>[13x]MAFLGAAIAAGLAAVAGAIAVAIIVKATIEGTTRQPELRGTLQTLMFIGVPLAEAVPIIAIVISLLILF

Most living cells depend upon the adenosine triphosphate (ATP) generated by F1Fo-ATP synthases that are energized by a proton- or a sodium-motive force (pmf, smf). Energetically down-hill ion translocation across the membrane through the Fo complex is mediated by successive interactions between the stator a-subunit and a rotor ring (c-ring). Translocation involves ion binding to an unoccupied c-subunit, rotation, and subsequent ion release. The c-ring is attached to the γε stalk subunits so that c-ring rotation causes rotation of the stalk.

We solved the crystal structure of a novel type of c-ring isolated from Bacillus pseudofirmus OF4 at 2.5 Å, revealing a cylinder with a tridecameric stoichiometry, a central pore, and an overall shape that is distinct from those reported thus far. In contrast with the distinctly hour-glass shape of the c11, K10, and c15 rotor rings, this c13 ring resembles a “tulip beer glass” appearance, in which the only slightly curved periplasmic side transitions at about the depth of the ion-binding site into a more significantly flared cytoplasmic side. While the inner helices are remarkably straight and only slightly tilted by ∼5° toward the c-ring axis (as seen from the periplasm), the outer helices are more curved and have a kink in the middle of the helix at the key carboxylate residue (Glu54). The more relaxed positioning of the helices in the alkaliphile ring is caused by the structural impact of the alanine motif AxAxAxA that replaces the glycine motif GxGxGxG most often found in the first helix coding region of c-subunits. On the outer helices of the c13 ring from an alkaliphile, two prolines located one helix turn below and above the ion-binding glutamate can be identified in a motif (PxxExxP) in which the first proline, Pro51, is specific for alkaliphiles. Within the groove of two neighboring c-subunits, the conserved glutamate of the outer helix shares the proton with a bound water molecule which itself is coordinated by three other amino acids of outer helices. One of these belongs to the side chain carboxyl oxygen (Oε2) of Glu54, whereas the three others originate from the backbone carbonyls of Leu52 and Ala53 and from the backbone nitrogen of Val56. However, several lines of evidence indicate the density seen in the binding pocket of this c13 ring should be interpreted as water rather than Na+. In contrast to other rotor ring structures, no residues from the inner helices contribute to ion coordination in the c13 ring. Although none of the inner helices contributes to ion binding and the glutamate has no other hydrogen bonding partner than the water oxygen, the site remains in a stable, ion-locked conformation that represents the functional state present at the c-ring/membrane interface during rotation.>[2x]SNAMRAVIPYKKAGAKSRLSPVLSLQEREEFVELMLNQVISSLKGAGIEQVDILSPS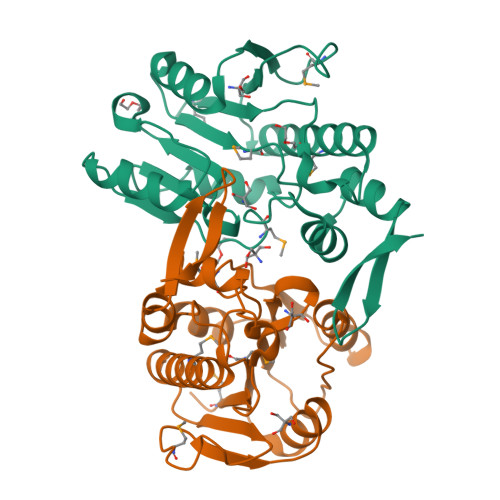VYGLEEMTEARVLLDEKDLNEALNRYLKEAEEPVLIVMADLPLLSPEHIKEISSTEKDVCIVPGKGGGTNALFIKNPSKYRVKYYGSSFLTHCSIATDSGQDFEIYDSFMAGTDIDEPEDLVELLIHGKGAAKDYIESKFRLEVKKGRVGLVPL>MKIFLDTANIDEIRTGVNWGIVDGVTTNPCLISKEAVNGKKYGDIIREILKIVDGPVSVEVVSTKYEGMVEEARKIHGLGDNAVVKIPMTEDGLRAIKTLSSEHINTNCTLVFNPIQALLAAKAGVTYVSPFVGRLDDIGEDGMQIIDMIRTIFNNYIIKTQILVASIRNPIHVLRSAVIGADVVTVPFNVLKSLMKHPKTDEGLAKFLECWKKVSPDGK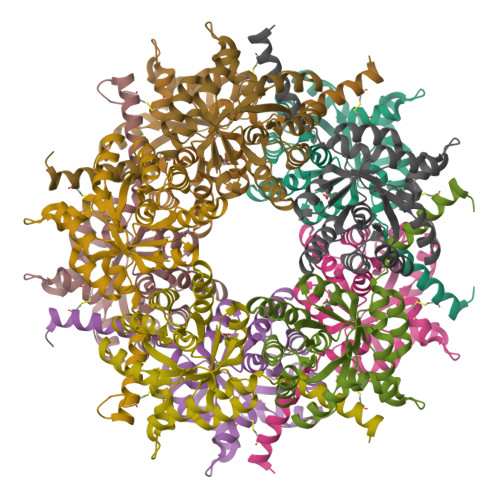LIL[5x]> LSTELSTE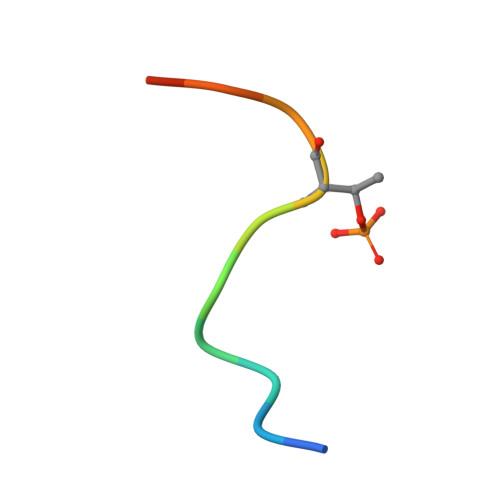PPSS>[2x]MVKFLGAVPVLTAVDVPANVSFWVDTLGFEKDFGDRD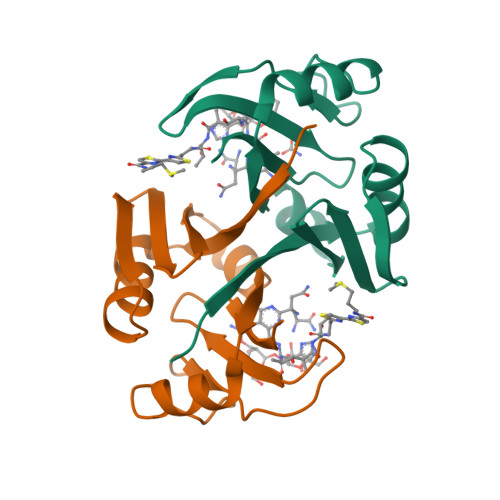FAGVRRGDIRLHISRTEHQIVADNTSAWIEVTDPDALHEEWARAVSTDYADTSGPAMTPVGESPAGREFAVRDPAGNCVHFTAGE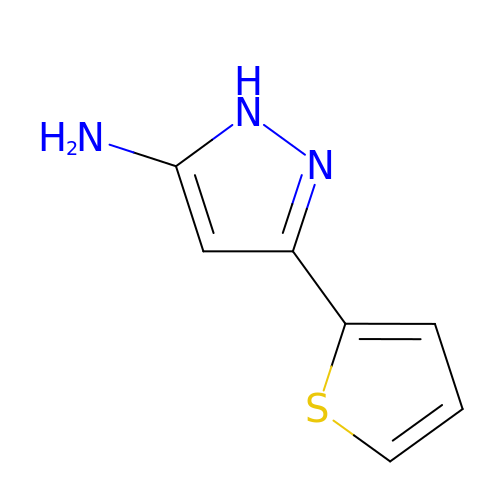3-thiophen-2-yl-1H-pyrazol-5-amine | C7 H7 N3 S | NPCGWFCMHOFZHD-UHFFFAOYSA-N> MRIHFILHETFEAPGAYLAWAALRGHDVSMTKVYRYEKLPKDIDDFDMLILMGGPQSPSSTKKEFPYYDAQAEVKLIQKAAKSEKIIVGVCLGAQLMGVAYGADYLHSPKKEIGNYLIS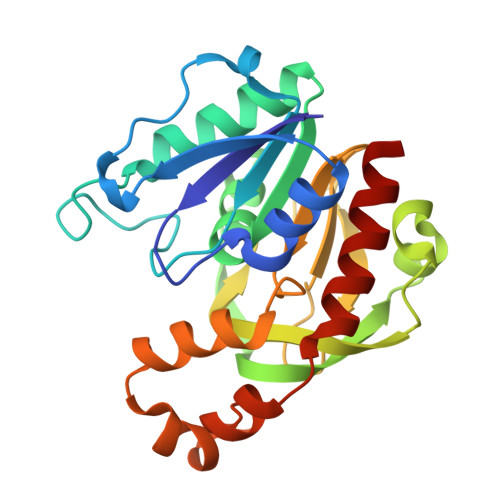LTEAGKMDSYLSDFSDDLLVGHWHGDMPGLPDKAQVLAISQGCPRQIIKFGPKQYAFQCHLEFTPELVAALIAQEDDLDTQSQTETYVQTAEEMQTFDYSSMNQALYSFLDRLTERK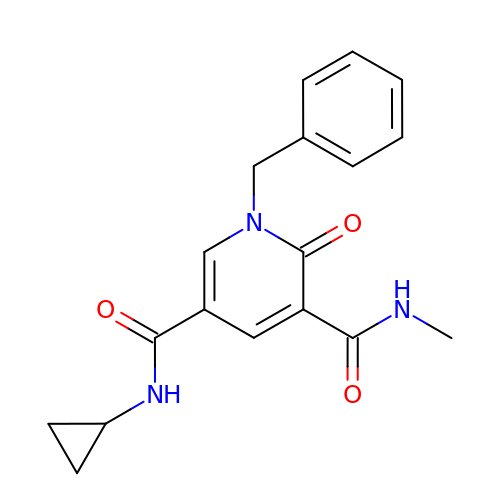~{N}5-cyclopropyl-~{N}3-methyl-2-oxidanylidene-1-(phenylmethyl)pyridine-3,5-dicarboxamide | C18 H19 N3 O3 | QZZCUOVXHPAQRQ-UHFFFAOYSA-N>CPSRCSCSGTTVECYSQGRTSVPTGIPAQTTYL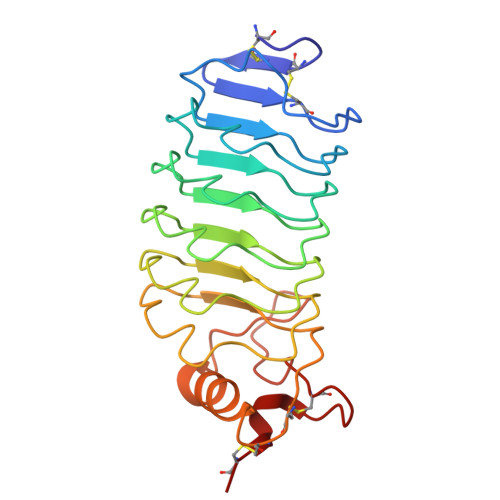DLETNSLKSLPNGVFDELTSLTQLYLGGNKLQSLPNGVFNKLTSLTYLNLSTNQLQSLPNGVFDKLTQLKELALNTNQLQSLPDGVFDKLTQLKDLRLYQNQLKSVPDGVFDRLTSLQYIWLHDNPWDCTCPGIRYLSEWINKHSGVVRNSAGSVAPDSAKCSGSGKPVRSIICP[2x]> M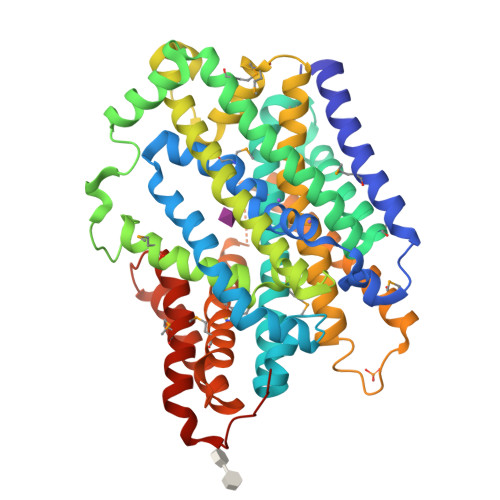QLHDFGFINYAVLFGYLAAMLLVGVYFSKRQKTADDYFRGGGRVPGWAAGVSVFATTLSSITFMSIPAKAYTSDWTFIIGQYLAIAILPLVFYFYIPFFRKLKITSAYEYLEARFDVRSRLFASLSFMLFHIGRVAIITYLTVLALRPFMGIDPVVLIVLISLLCIIYTWMGGIEGVIWTDVIQGLLLSGGAVLIFIMICFKVDGGISEIFTTTAQADKFFPTTQWRWSWTDSTIPVLMIGFLFANIQQFTASQDVVQRYIVTDSIKETKRTLITNAKLVAIIPIFFFAIGSALFVYYQQNPSLLPAGFNTGGILPLFIVTEMPIGIAGLIIAAIFAAAQSSISSSLNSISSCFNSDIYTRLSKSSPSPEQKMKVAKLVIIVAGIFSSLAAIWLVLSDEAEIWDAFNSLIGLMGGPMTGLFMLGIFVKRANAGSAVVGIIVSIIAVLAARYGSDLNFFFYGVIGSMSVVIAGTITAPLFAPAKQLSLDDSETSEN>[4x]MIKQAVILAGGLGSRLK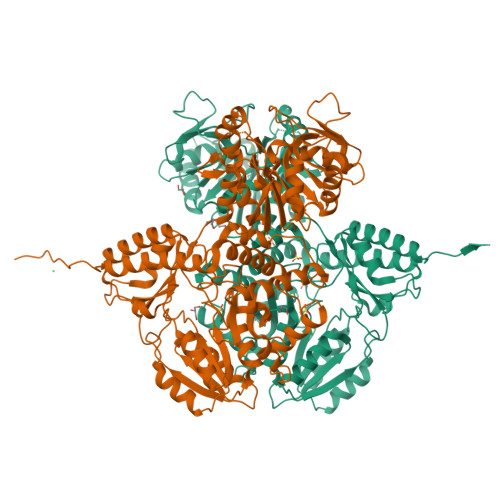DKTKTMPKGFLEIGGTAIVEQSVQKLLAHGIEKIVIGTGHCNEYYDNLAKKYPAIITVKNENYANTGSMGTLEVCASFVNESFLLLESDLIYDSAGLFSLINDERKNLILASGATKSGDEVYLEADEKNCLTGLSKNRDALKNIFGELVGITKLTKSTLDKMCAYAKIHHSDLPKMEYEHALLEAAKTIPVAIKRIEYFVWREIDNEDHLEMAVKNIYPHIVENEKLRAVRREVLLNPGPATTTDSVKYAQVSADICPREKAFGDLMQWLCDELKLFALASETNPDEYETVMFGCSGTGADEVMVSSCVPDTGRLLVIDNGSYGARMAKIADIYKIPMDIFKSSTYEPLDLQKLEAEFATKKYTHLACVYHETTTGLLNPLHIICPMAKKYGMVTIVDAVSAYCGMPMDLKSLGIDFMASTSNKNIQGMAGVGFVICNKAELEKTKDYPMRNYYLNLYDQYAYFAKTHQTRFTPPVQTMYALRQAVLETKQETVQKRYERYTACWNILVAAIKKLGLKMLVKEEHQSHFITAILEPETPKYSFEALHDFAAEHSFTIYPGKLGNIDTFRIANIGDIQPEEMRRFTVKLKEYMNGIGVGVLEHHHHHH>MTTLQEKIIQELGVLPTIDPKEEVRKSIDFLKAYLTKHPFLKTFVLGISGGQDSTLAGRLAQLAMTEMREETGDMSYQFIAIRLPYGEQADEADAQAALAFIQPDVSLRVDIKP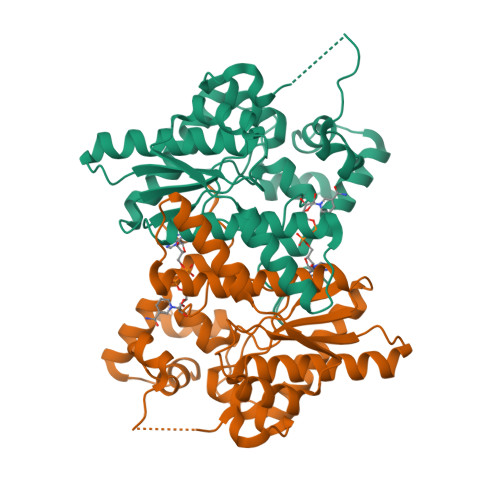AVDAMVGSLENAGVQISDFNKGNMKARQRMITQYAVAGENAGAVIGTDHAAENVTAFFTKYGDGGADILPLFRLNKRQGKALLKELGAPEALYLKIPTADLEDDKPLVADEVALGVTYDAIDDYLEGKKVSETDQQTIENWYKKGQHKRHLPITIFDDFWK[8x]Thiol dioxygenases are a subset of nonheme iron oxygenases that catalyze the formation of sulfinic acids from sulfhydryl-containing substrates and dioxygen. Av3MDO exhibits the classic thiol dioxygenase cupin fold consisting of three N-terminal alpha-helices followed by a series of 11 β-strands forming the cupin β-barrel structure that houses the enzymatic active site. Like in Pa3MDO and other thiol dioxygenases, the iron center of Av3MDO is coordinated by three His residues (90, 92, and 142) contained within the conserved cupin motifs. The moderately hydrophobic dimer interface buries an average of ∼1260 Å2 (1199–1322 Å2 depending on the specific dimer pair) or ∼13% of the total monomer surface area and is structurally similar to the dimers observed for 3MDOs from other bacteria, all suggesting that it represents a physiologically relevant assembly.

The optimized crystals diffracted X-rays to ∼2.2 Å resolution and belonged to space group P31. The asymmetric unit of the Av3MDO crystals consists of 12 monomers arranged in pairs of C2 symmetric dimers. Analysis of residual electron density maps revealed two strong features near the Av3MDO iron center, which could not be successfully modeled with aquo ligands as was the case for Pa3MDO. A chloride ligand was bound to iron in the coordination site assigned as the O2-binding site. Chloride binds to the iron center trans to His90 at a distance of ∼2.4 Å and simultaneously contacts the hydroxyl moiety of Tyr159 forming a 2.7 Å ion–dipole interaction. The carboxylate group simultaneously engages in an ionic interaction with Arg168, which is situated adjacent to the iron center. However, inspection of the Av3MDO structure revealed that its active site is completely sealed off to the bulk solvent (left). In comparison to the homologous residues of Pa3MDO, residues Tyr61, Pro88, and Phe180 of Av3MDO are shifted inward toward each other to occlude the potential passageway. Notably, the difference in Trp81 rotameric state results in different arrangements of the “SHY” motif between Av3MDO and Pa3MDO. In combination with spectroscopic simulations and optimized DFT models, this work provides an experimentally verified model of the Av3MDO enzyme–substrate complex, effectively resolving a debate in the literature regarding the preferred substrate-binding denticity.

>MSESPLRLDRLRDFVSALGELLDRHPDEESVLREGRSLLGELVRHDDWLPEEFAQPDPERYQQYLLHADSRQRFSVVSFVWGPGQTTPVHDHRVWGLIGMLRGAEDAQSFELGAEGLRPIGDPVRLSPGQVEAVSPRIGDIHRVFNASPDQPSISIHVYGANIGAVRRAVYLPDGSEKPFISGYSNQFLPNIWDQSKESARPVDLVPR[12x]>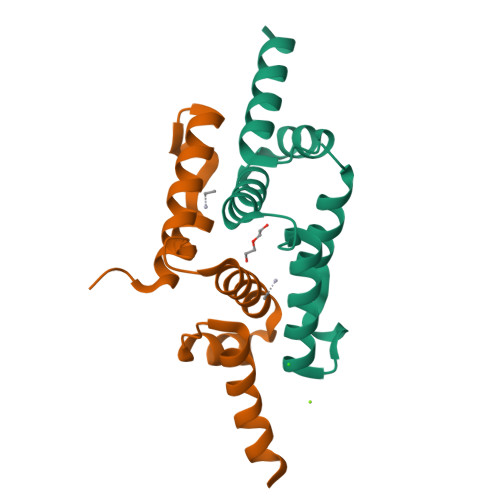[2x]GSPDPEIFRQRFRQFGYQDSPGPREAVSQLRELCRLWLRPETHTKEQILELVVLEQFVAILPKELQTWVRDHHPENGEEAVTVLEDLESELDD>MAHHHHHHGSMPISKIHARSVYDSRGNPTVEVDVVTETGLHRAIVPSGASTGQHEAHELRDGDKTQWGGKGVLKAVKNVNETIGPALIKENIDVKDQSKVDEFLNKLDGTANKSNLGANAILGVSLAVAKAGAAEKGVPLYAHISDLAGTKKPYVLPVPFQNVLNGGSHAGGRLAFQEFMIVPDSAPSFSEALRQGAEVYQKLKALAKKKYGQSAGNVGDEGGVAPDIQTAEEALDLITEAIEQAGYTGKIKIAMDVASSEFYKADVKKYDLDFKNPESDPSKWLTYEQLADLYKSLAAKYPIVSIEDPFAEDDWEAWSYFYKTSDFQIVGDDLTVTNPGRIKKAIELKSCNALLLKVNQIGTLTESIQAAKDSYADNWGVMVSHRSGETEDVTI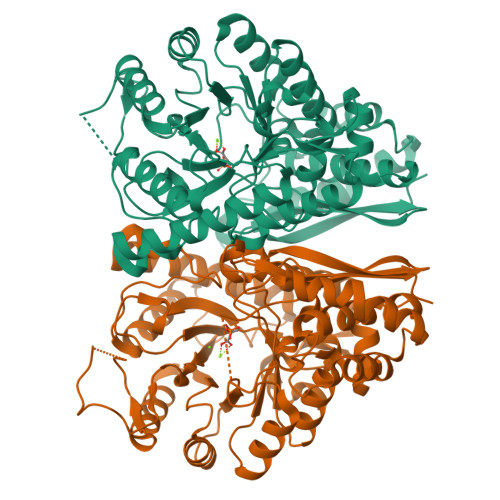ADIAVGLRSGQIKTGAPCRSERLAKLNQILRIEEELGENAVYAGSKFRTAVNL[2x]> MDVLEMFDVNYESPILESFDSTTQSLNDVHVFMSRIQMSAYDADGEGRIEYRNLKLYEISSGIFISTDRLDTGASGVEDDHEMVDYYSSARLTREFLGESLDSQKSDYFEGIKKVFSFYKNKCNESRYIKEFFEEIQFRNICGFPKQAGTSSTDIFDQFNSVDVLLQDPVTSVWNKKVGSKKANIVIIPPATNLPITEACATAGFQPEGFPKLGSGSFFTVQFDPFFSTRFKAHETDDVALLDPTLTLLHEMTHGLHFQKGIANPVNRSGETPAWATTWGRVTGDNDAFKETPMEELLTFNKHTIDDDIEISDHLKSTYIGFLYNGRNEDDPTESVDGVYQNVSSFLNQYRGFEISSDFQHFIESCYGVKYNQESKKFIVNPRNIKRYVQDGFFIDEAKFARILNIKTRSYYTLMPDNLGVWSYRVDILNRLRETFDEDRGLLSQELDFHTALTPVVSENPALELEVAGMQRMVSLPKIKASYLPSDIKIKNFTGQKISHDTILDTNISGIIISKIKYKSDFVVDESMPRSSLNTTNYNLSPIKGTKFETDIRDKTSVKVTVSEITAPMINHVMKLDNSKVLTERPSLNEDLEETFKNTKDVYIPKTTAMMKLKEGADQTLGAVGFAVWSGQILEDLYNLAQKKEVSIDQIKDDLMSILPFYCAYKNLSAEKYEQAFANATLDAFLIFATDGGGFAGLGITVGAIAINSMYAKAETMEAYDSMFGKYVDQYQNDIKNFTLNAYVQWENNILSRLWNESRLAITGFRNMLKTVKTVMEFDATNQAYSEEDRKIIKAKCEEIFSEFPMLMQTFAKNSMTANLENASKIFNDIVWQKIKEELDQYVIDSKKYFLDSLEEAYNNGSISAESYYKYQTEAREKFVSPREVIDLYIAAHDTVVKRKRYIRRYSRKYDLATDFKGNTVHLNGLGEGTQDIQDLYGNYSVYADKKTVSTQEGHFDQTIKIAKDTNTINKVVLAVSSNNGKEYALNKDEQYTISFWLRMPVPSSSEERRIFSYSAVSGVNKEVEELILQVKNNEFVLATANLLRNSEFVIEPRIALNRWVKITIVNENTRIKVYQNDNLLGLIKDSSRKKPIAQRGTFKFYNYNVDYQLDDISYYNGTISQRDIKYTFKEDHGQFVYDHWGERLQYNKAYYLLSDDNKSAFETVYETKRLKLKSVPGVDIKYLGMNDRVYGYYGGLQFKLVPLDSKNMNNYVRWGDKFTMQSIETTNLSLAIIQDNAYFAPTQLKLISNEGKSEEEIFTFDRNIKLQNAAILVGTGNSKQGPISAYKRGYSGDLWINGARLDGYVTVVNKSNYSNDEIQEKFKWIFVPKDANWVEGSYPYDVPDYALESGKETAAAKFERQHMDSSTSAA;> MGSDYKDDDDKSGMDNKLKTENIRYFRTAAGSEDVLEVKAYEVYPNVWAIPSRYMMEPLQDLDEVTNPEQFSIYDKKYLADIQEQDEFLKSIQAAIEDIKKRTFGLELLTAVSGAVPLPKDTGATNTTLQCIDENGKHTHDVVANVVLWGPGNNLNSNRLISKSDDDSNGIGSMVELIWNPQILIKNIGTNRIKPATDELVGLLTKALFRLYGLGLNKIRYPFYQLDDKKYYSLTAEDLISYGGFSANVVNLQPYYFLEDQFTKVKEKYESAKKRIDDIKVNDEYSQMLTLKYQFDLYSLFHISTSYIVSTVIPANDKYGGLVSYYTGPNALIDSKTDEKLTSMVKIPLKKIKYSKNQSREYDEYDLTNGEDSTQYFENFTFPKSKHVFVETQPTPENVFVNLPSEEITKIILPVIPAESDLIKIPFQPATPKSITTELITTDVPTLGLIFPAVKSKQNLSDIKMTSKLSDALDSDKQTFAFDNTLVDKLSELTSVSDAELFGIIRLIKNELLSVIDNFTTFGDNWSCPRWIDYCFQQVFGSDLKNLIVQGDFEKVFNISDTLILPKQLPEDILQLKPYLFYQWYAKRYTR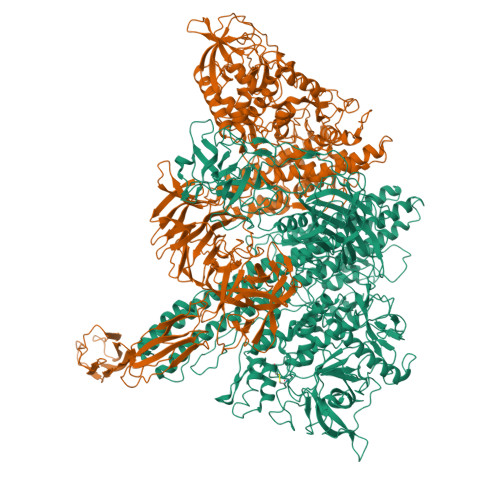ILRLESLFYQILNEHITLIRSLVSSNNKGQYLQGFMNDLDKIAYNAQYMLSDWTIQLGYYDFKNQVTQVIKTSSMTSEFNIDDLLYDYDTFKLTISQFGADSINNFTPSQDLKLALNDNNSPILLLGNDEIKSNGSITQTDDSLDDETSLLLSKNTSFEGNFSAKYLLSSVGVNFTFKSIENLNFSVDFMNINIAFSNNFFEITQTGQETKKYSIAKLFGWNSLVYLIKHSSVEIWDIHSNILLVSHDLTAPQNNIVKAPIKLTNLDNELILKSFEVFEQDEEANYNDIEQGFKNGIIYTAKKMPIIVGEKYALKSSILDDMGILTSDENKKYPVFSTDVEVESSLNIILESTTGDKISVDAGVNIRTINSNGEENYLGIEDNHLIFVPKEEAELFYLKKAVVEDTIDIFYVVKTLGNMFINVERISDNIYRLNFKAGILYSTMESDMLVLPAEEANTAFYIQPIGLASLEVKDSVLGEGNPWLKEDNFLDATDDYGNQIDLSDNRISVTGSVDTDKVGTYSVVYSYTGIDKTNTEKATITVKLDKSSIKTQDSTLQNGKEWVRADNLVEVIDEDGNKVDYSDDRIIQEGDVDINKAGVYDITFRYRGKFKIISSSFKVTVINDIWYDSIKNACKTYLIDYGERINDVKGITFQNILEATRGKLYGYRVVYDNPHDVINQNPPKDFHFDLIKPFDVKNPSRVHLADYSGYLRLFIISTGKINTDIKVKIYAVLENKDEIEIFDNHQNDKRHEEIAEIYKSNFDDNNYSADGKYFISVLFKNDVQAVVKDEIYGYEIFYSYFTKFRKDTAFQTDGSKRIFFHDYFNFEVPLDYKDSTFINVILKNGEKIRIYKFAGYYYYSGHHHHHH> MSLRTGKTNVIALVLSVDEELMGFTSQMVFGITEVLSTTQYHLVVTPHIHAKDSMVPIRYILETGSADGVIISKIEPNDPRVRFMTERNMPFVTHGRSDMGIEHAFHDFDNEAYAYEAVERLAQCGRKRIAVIVPPSRFSFHDHARKGFNRGIRDFGLTEFPIDAVTIETPLEKIRDFGQRLMQSSDRPDGIVSISGSS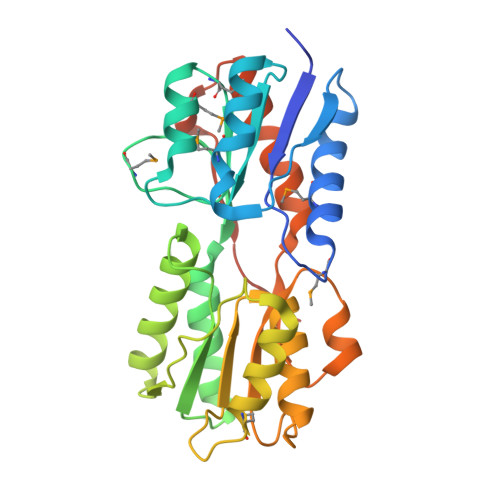TIALVAGFEAAGVKIGEDVDIVSKQSAEFLNWIKPQIHTVNEDIKLAGRELAKALLARINGEAAETLQSISGPVWSSMAPKEGHHHHHH(3AR,5R,6S,7R,7AR)-2-(ETHYLAMINO)-5-(HYDROXYMETHYL)-5,6,7,7A-TETRAHYDRO-3AH-PYRANO[3,2-D][1,3]THIAZOLE-6,7-DIOL 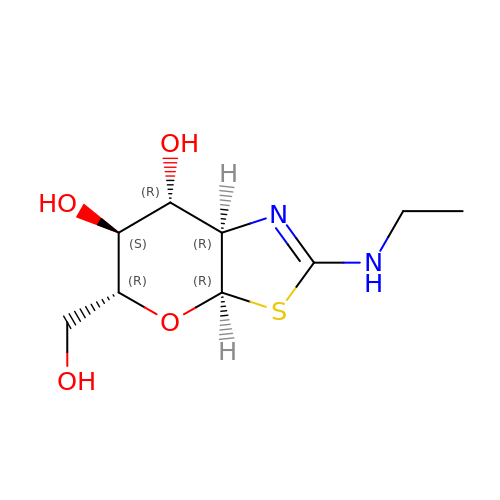| C9 H16 N2 O4 S | PPAIMZHKIXDJRN-FMDGEEDCSA-N> FRAIIESPEGAGHVGYQYRRNTGSTMRMVSDVLDERVSLWDFHCDPSGNVIQPGPNVDSRQYLQAAIDYVSSNGGGTITIPAGYTWYLGSYGVGGIAGHSGIIQLRSNVNLNIEGRIHLSPFFDLKPFQVFVGFDNGDPASSGNLENCHIYGHGVVDFGGYEFGASSQLRNGVAFGRSYNCSVTGITFQNGDVTWAITLGWNGYGSNCYVRKCRFINLVNSSVNANHSTVYVNCPYSGVESCYFSMSSSFARNIACSVQLHQHDTFYRGSTVNGYCRGAYVVMHAAEAAGAGSYAYNMQVENNIAVIYGQFVILGSDVTATVSGHLNDVIVSGNIVSIGERAAFSAPFGAFIDIGPDNSGASNVQDIQRV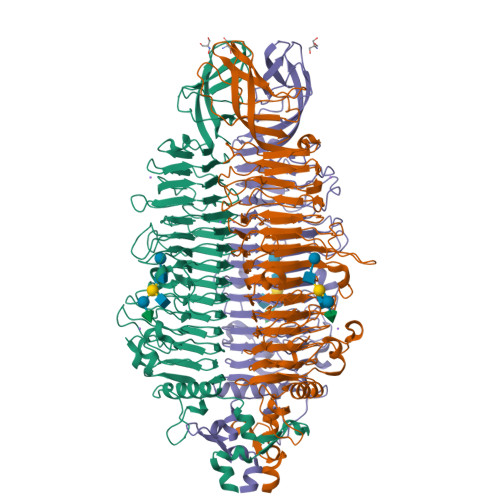LVTGNSFYAPANITDSAAITLRANLNGCTFIANNFDCRYMVYNAPGTTSPVVQNLVWDKSNVIGGTHANQRAGQNLFDMQFASVVNSTIEVQLSCEDLSMFSCILFPASCQLSYSKITVDSAWTKSMSNTAVFEGNQQAGANVYVSYPATVNLTSYNTQGAVPFFSTDTNYAWVTSAYSLSINENLDFSPPATYTNKANGQLVGVGYNEIGGVRSVSVRLMLQRQV>[2x]GUGUGAGGCUG;>[2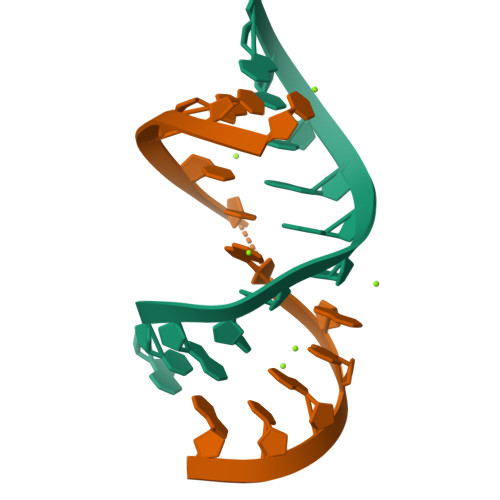x]CCAGUCGGAACA>GAMGSEPRPTAPSSGAPGLAGVGETPSAAALAAARVELPGTAVPSVPEDAAPASRDGGGVRDEGPAAAGDGLGRPLGPTPSQSRFQVDLVSENAGRAAAAAAAAAAAAAAAGAGAGAKQTPADGEASGESEPAKGSEEAKGRFRVNFVDPAASSSAEDSLSDAAGVGVDGPNVSFQNGGDTVLSEGSSLHSGGGGGSGHHQHYYYDTHTNTYYLRTFGHNTMDAVPRIDHYRHTAAQLGEKLLRPSLAELHDELEKEPFEDGFANGEESTPTRDAVVTYTAESKGVVKFGWINGVLVRCMLNIWGVMLFIR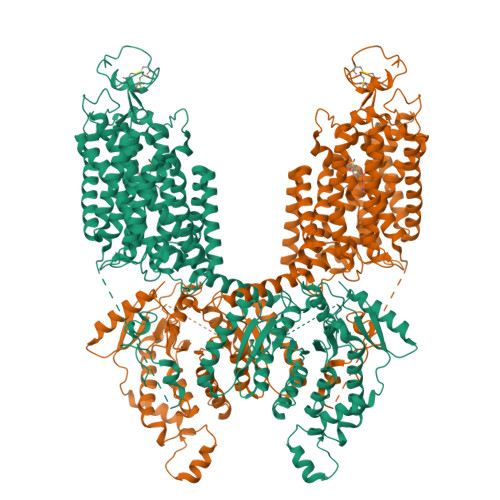LSWIVGQAGIGLSVLVIMMATVVTTITGLSTSAIATNGFVRGGGAYYLISRSLGPEFGGAIGLIFAFANAVAVAMYVVGFAETVVELLKEHSILMIDEINDIRIIGAITVVILLGISVAGMEWEAKAQIVLLVILLLAIGDFVIGTFIPLESKKPKGFFGYKSEIFNENFGPDFREEETFFSVFEIFFPAATGILAGANISGDLADPQSAIPKGTLLAILITTLVYVGIAVSVGSCVVRDATGNVNDTIVTELTNCTSAACKLNFDFSSCESSPCSYGLMNNFQVMSMVSGFTPLISAGIFSATLSSALASLVSAPKIFQALCKDNIYPAFQMFAKGYGKNNEPLRGYILTFLIALGFILIAECNVIAPIISNFFLASYALINFSVFHASLAKSPGWRPAFKYYNMWISLLGAILCCIVMFVINWWAALLTYVIVLGLYIYVTYKKPDVNWGSSTQALTYLNALQHSIRLSGVEDHVKNFRPQCLVMTGAPNSRPALLHLVHDFTKNVGLMICGHVHMGPRRQAMKEMSIDQAKYQRWLIKNKMKAFYAPVHADDLREGAQYLMQAAGLGRMKPNTLVLGFKKDWLQADMRDVDMYINLFHDAFDIQYGVVVIRLKEGLDISHLQGQEELLSSQEKSPGTKDVVVSVEYSKKSDLDTSKPLSEKPITHKVEEEDGKTATQPLLKKESKGPIVPLNVADQKLLEASTQFQKKQGKNTIDVWWLFDDGGLTLLIPYLLTTKKKWKDCKIRVFIGGKINRIDHDRRAMATLLSKFRIDFSDIMVLGDINTKPKKENIIAFEEIIEPYRLHEDDKEQDIADKMKEDEPWRITDNELELYKTKTYRQIRLNELLKEHSSTANIIVMSLPVARKGAVSSALYMAWLEALSKDLPPILLVRGNHQSVLTFYS[2x]> DLGAPQNPNAKAAGSRKIHFNWLPPSGKPMGYRVKYWIQGD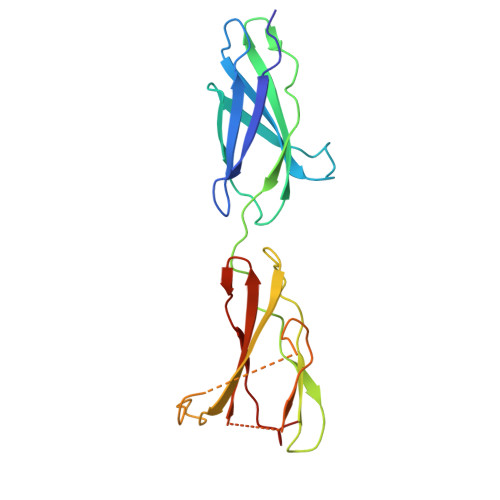SESEAHLLDSKVPSVELTNLYPYCDYEMKVCAYGAQGEGPYSSLVSCRTHQEVPSEPGRLAFNVVSSTVTQLSWAEPAETNGEITAYEVCYGLVNDDNRPIGPMKKVLVDNPKNRMLLIENLRESQPYRYTVKARNGAGWGPEREAIINLATQP>MNPAAEAEFNILLATDSYKVTHYKQYPPNTSKVYSYFECREKKTENSKLRKVKYEETVFYGLQYILNKYLKGKVVTKEKIQEAKDVYKEHFQDDVFNEKGWNYILEKYDGHLPIEIKAVPEGFVIPRGNVLFTVENTDPECYWLTNWIETILVQSWYPITVATNSREQKKILAKYLLETSGNLDGLEYKLHDFGYRGVSSQETAGIGASAHLVNFKGTDTVAGLALIKKYYGTKDPVPGYSVPAAEHSTITAWGKD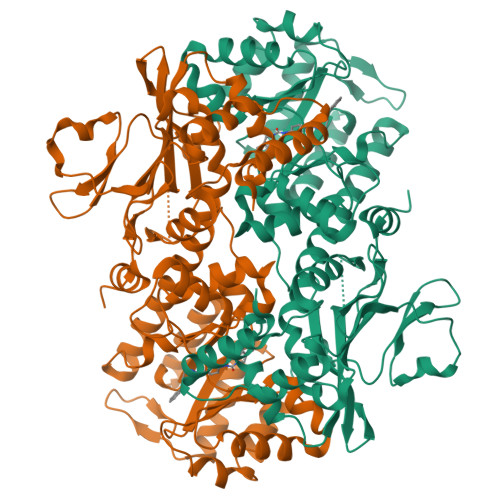HEKDAFEHIVTQFSSVPVSVVSDSYDIYNACEKIWGEDLRHLIVSRSTQAPLIIRPDSGNPLDTVLKVLEILGKKFPVTENSKGYKLLPPYLRVIQGDGVDINTLQEIVEGMKQKMWSIENIAFGSGGGLLQKLTRDLLNCSFKCSYVVTNGLGINVFKDPVADPNKRSKKGRLSLHRTPAGNFVTLEEGKGDLEEYGQDLLHTVFKNGKVTKSYSFDEIRKNAQLNIELEAAHHDYKDDDDK[2x]> HHHHHHSGSGENLYFQGSGSEEIVEEAETALKALLEEAEKGGKEDALEIAEKLAELAKEALEVLLEAGASPELIVRLAETALKALLAIAELGGEELALEIARILAELAEVALEVLLELGASPELIVRLAETALEALLAIARLGGEELALEIARILAELAEVALEVLLELGASPELIKKLAETAEEALEAIAKLGGEELAEEIAKILAELAEVAKE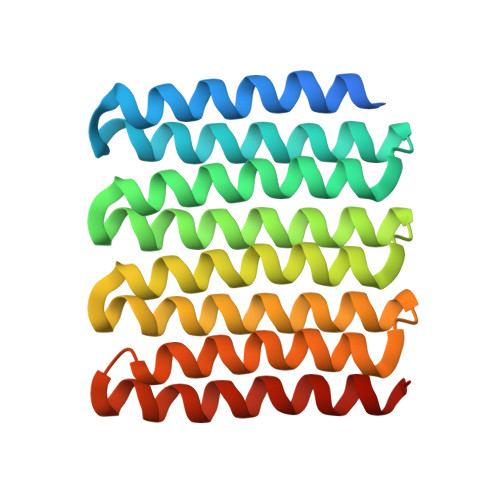VQKELGAS> MGSDKIHHHHHHMPKSVRAENISRILKRIMKSPVSRVEL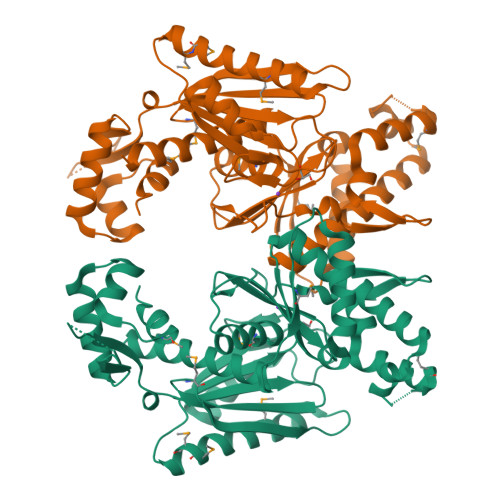AEELGLTKTTVGEIAKIFLEKGIVVEEKDSPKGVGRPTKSLKISPNCAYVLGIEVTRDEIAACLIDASMNILAHEAHPLPSQSDREETLNVMYRIIDRAKDMMEKLGSKLSALTVAAPGPIDTERGIIIDPRNFPLSQIPLANLLKEKYGIEVWVENDADMGAVGEKWYTKRDDSFAWILTGKGIGAGIIIDGELYRGENGYAGEIGYTRVFNGNEYVFLEDVCNENVVLKHVLSMGFSSLAEARDSGDVRVKEYFDDIARYFSIGLLNLIHLFGISKIVIGGFFKELGENFLKKIKIEVETHLLYKHSVDMSFSKVQEPVIAFGAAVHALENYLERVTTS> MGLEKTVKEKLSFEGVGIHTGEYSKLIIHPEKEGTGIRFFKNGVYIPARHEFVVHTNHSTDLGFKGQRIKTVEHILSVLHLLEITNVTIEVIGNEIPILDGSGWEFYEAIRKNILNQNREIDYFVVEEPIIVEDEGRLIKAEPSDTLEVTYEGEFKNFLGRQKFTFVEGNEEEIVLARTFAFDWEIEHIKKVGLGKGGSLKNTLVLGKDKVYNPEGLRYENEPVRHKVFDLIGDLYLLGSPVKGKFYSFRGGHS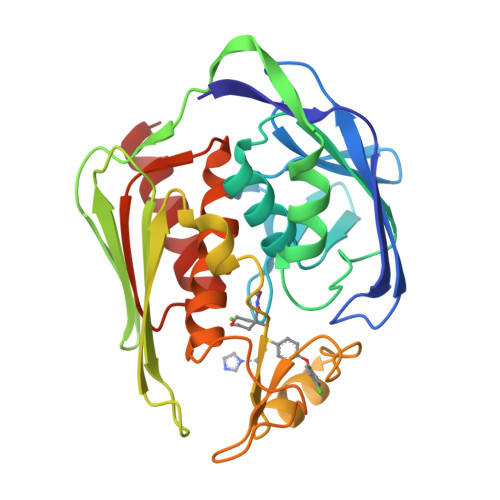LNVKLVKELAKKQKLTR>[4x]TMQGFGVHTSMWTMNWDRPGAERAVAAALKYEVDFIEIPMLNPPAVDTEHTRALLEKNELRALCSLGLPE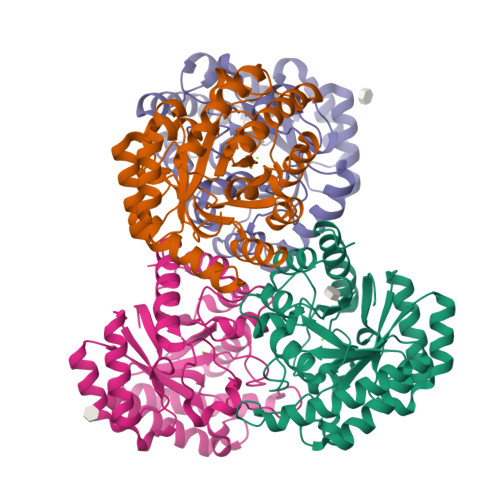RAWASVRPDAAIEHLKVAIDKTADLGGEALSGVIYGGIGERTGVPPTEAEYDNIARVLSAAAKHAKSRGIELGVEAVNRYENHLINTGWQAVQMIERVGADNIFVHLDTYHMNIEEKGVGNGILDAREHLKYIHLSESDRGTPGYGTCGWDEIFSTLAAIGFKGGLAMESFINMPPEVAYGLAVWRPVAKDEEEVMGNGLPFLRNKAKQYGLI> ATCDDGRTTANAACCILFPILDDIQENLFDGAQCGEEVHESLRLTFHDAIGFSPTLGGG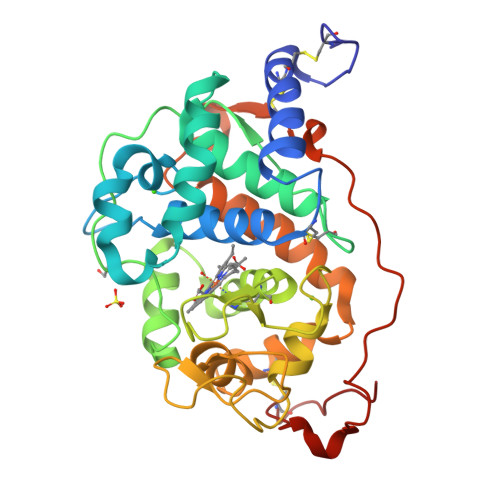GADGSIIAFDTIETNFPANAGIDEIVSAQKPFVAKHNISAGDFIQFAGAVGVSNCPGGVRIPFFLGRPDAVAASPDHLVPEGFDSVDSILARMGDAGFSPVEVVWLLASHSIAAADKVDPSIPGTPFDSTPEVFDSQFFIETQLKGRLFPGTADNKGEAQSPLQGEIRLQSDHLLARDPQTACEWQSMVNNQPKIQNRFAATMSKMALLGQDKTKLIDCSDVIPTPPALVGAAHLPAGFSLSDVEQACAATPFPAL>[2x]MADDQGCIEEQGVEDSANEDSVDAKPDRSSFVPSLFSKKKKNVTMRSIKTTRDRVPTYQYNMNFEKLGKCIIINNKNFDKVTGMGVRNGTDKDAEALFKCFRSLGFDVIVYNDCSCAKMQDLLKKASEEDHTNAACFACILLSHGEENVIYGKDGVTPIKDLTAHFRGDRCKTLLEKPKLFFIQACRGTELDDGIQAD;>SGPINDTDANPRYKIPVEADFLFAYSTVPGYY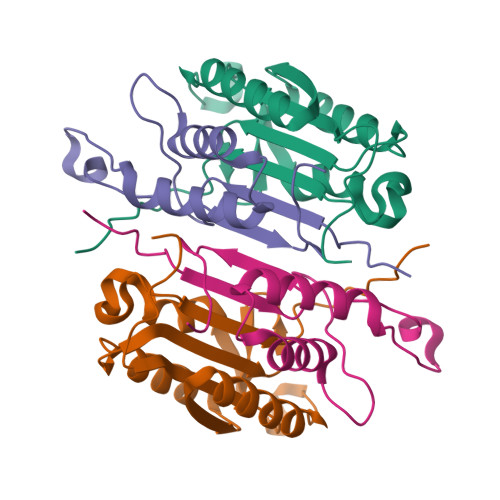SWRSPGRGEWFVQALCSILEEHGKDLEIMQILTRVNDRVARHFESQSDDPHFHEKKQIPCVVSMLTKELYFSQLEHHHHHH[2x]> MEGFIQNKRKKEKEGEEEEESKEKRKQINQLNKQKQEEEKIYQQKKDQKRKKYLYQRKEMTIFAETWEASEYQYRNKANLKTLPVNHLGKLAELKFDFVEYKAHQLIAC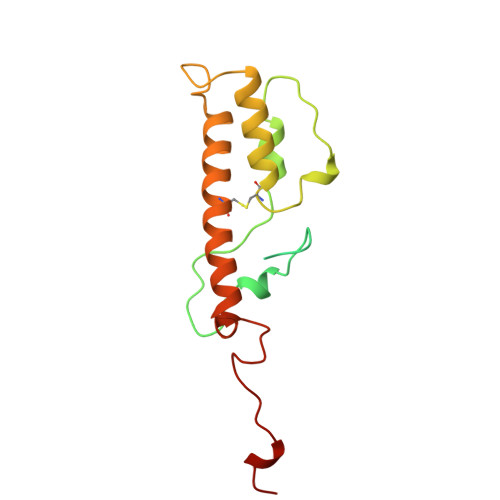HLYERMTIHCMNQYGLFKDFYRPECLDAQYYFKTCVELNAAYGIQKKFFPEHFVGSPYARPVPQFQQLGL>MTFERNKTLYWGGALWSPPSNWNPFTPWNAVAGTIGLVYEPLFLYDPLNDKFEPWLAEKGEWVSNNEYVLTLRKGLRWQDGVPLTADDVVFTFEIAKKYTGISYSPVWNWLGRIERVDERTLKFVFSDPRYQEWKQMLINTPIVPKHIWENKTEEEVLQAANENPVGSGPYYVESWADDRCVFKKNGNWWGIRELGYDPKPERIVELRVLSNNVAVGMLMKGELDWSNFFLPGVPVLKKAYGIVTWYENAPYMLPANTAGIYINVNKYPLSIPEFRRAMAYAINPEKI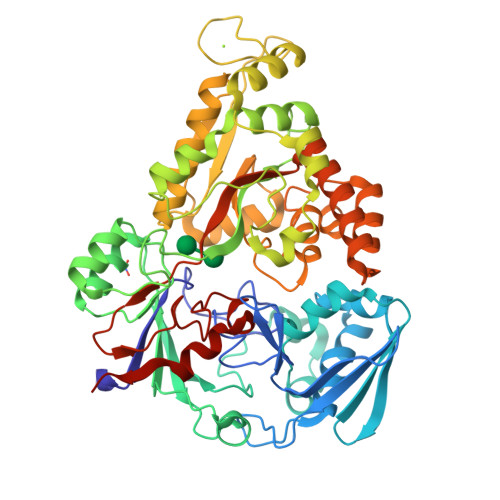VTRAYENMVTAANPAGILPLPGYMKYYPKEVVDKYGFKYDPEMAKKILDELGFKDVNKDGFREDPNGKPFKLTIECPYGWTDWMVSIQSIAEDLVKVGINVEPKYPDYSKYADDLYGGKFDLILNNFTTGVSATIWSYFNGVFYPDAVESEYSYSGNFGKYANPEVETLLDELNRSNDDAKIKEVVAKLSEILLKDLPFIPLWYNGAWFQASEAVWTNWPTEKNPYAVPIGWNGWWQLTGIKTLFGIEAKHHHHHH[2x]> AEQKTLHIYNWTDYIAPDTVANFEKETGIKVVYDVFDSNEVLEGKLMAGSTGFDLVVPSAYLLERQLTAGVFQPLDKSKLPEWKNLDPELLKLVAKHDPDNKFAMPYMWATTGIGYNVDKVKAVLGENAPVDSWDLILKPENLEKLKSCGVSFLDDPEEVFATVLNYLGKDPNSTKADDYTGPATDLLLKLRPN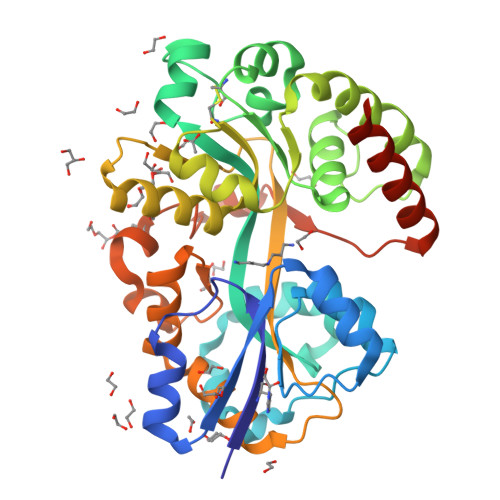IRYFHSSQYINDLANGDICVAIGWAGSVWQASNRAKEAKNGVNVSFSIPKEGAMAWFDVFAMPADAKNKDEAYQFLNYLLRPDVVAHISDHVFYANANKAATPLVSAEVRENPGIYPPADVRAKLFTQKVQDPKIDRVRTRAWTKVKSGKLEHHHHHH>[2x]MHHHHHHDEKRENDPAKVKEAILAAKAAGRSRKDGNLERAMTIMEHAMALAPTNPQILIEMGQIREMHNELVEADQCYVKALAYDPGNSEALVLRARTTPLVSAIDRKMLRSVHDLRDEFNHLQHSTALRRMMRETYFLYVYHTVAIGGNTLSLGQTRAILESGMVIPGKSIREHNEVIGMDAALRFLNCSLLSKEHDE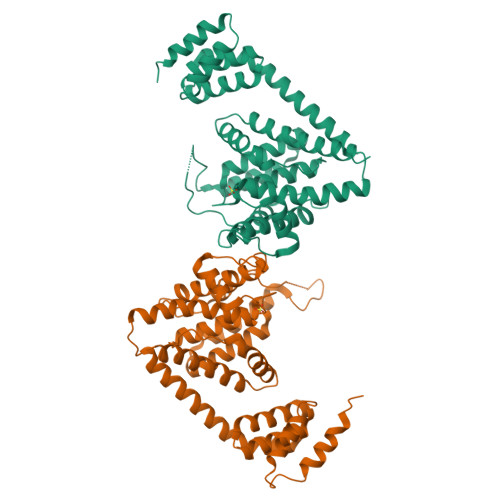ISIDDILEMHRRVLGNADPVEAGRIRTTQVYVGRFTPVSPEYVMEQLKDIVDWLNDESTLTIDPIERAAIAHYKLVLVHPFTDGNGRTARLLLNLIMMRSGFPPVILPVETRAEYYASLHVANLGDLRPFVRYVAKHSEASIQRYIGAMKTSSDNILNSGDSKLTPEESEVSEKIEAECRAGN>C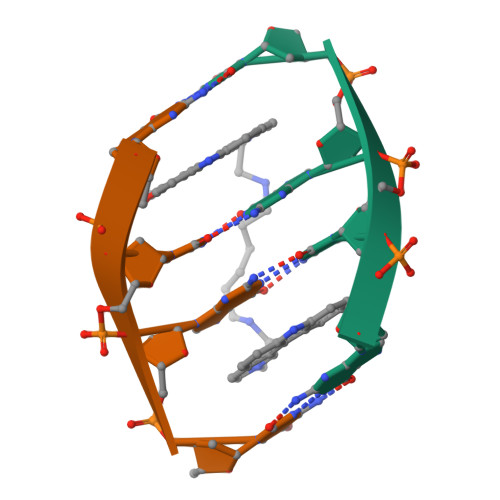GCG[2x]>MESEQLFHRGYYRNSYNSITSASSDEELLDGAGAIMDFQTSEDDNLLDGDTAAGTHYTMTNGGSINSSTHLLDLLDEPIPGVGTYDDFHTIDWVREKCKDRERHRRINSKKKESAWEMTKSLYDAWSGWLVVTLTGLASGALAGLIDIAADWMTDLKEGICLSALWYNHEQCCWGSNETTFEERDKCPQWKTWAELIIGQAEGPGSYIMNYIMYIFWALSFAFLAVSLVKVFAPYACGSGIPEIKTILSGFIIRGYLGKWTLMIKTITLVLAVASGLSLGKEGPLVHVACCCGNIFSYLFPKYSTNEAKKREVLSAASAAGVSVAFGAPIGGVLFSLEEVSYYFPLKTLWRSFFAALVAAFVLRSINPFGNSRLVLFYVEYHTPWYLFELFPFILLGVFGGLWGAFFIRANIAWCRRRKSTKFGKYPVLEVIIVAAITAVIAFPNPYTRLNTSELIKELFTDCGPLESSSLCDYRNDMNASKIVDDIPDRPAGVGVYSAIWQLCLALIFKIIMTVFTFGIKVPSGLFIPSMAIGAIAGRIVGIAVEQLAYYHHDWFIFKEWCEVGADCITPGLYAMVGAAACLGGVTRMTVSLVVIVFELTGGLEYTVPLMAAVMTSKWVGDAFGREGIYEAHIRLNGYPFLDAKEEFTHTTLAADVMRPRRSDPPLAVLT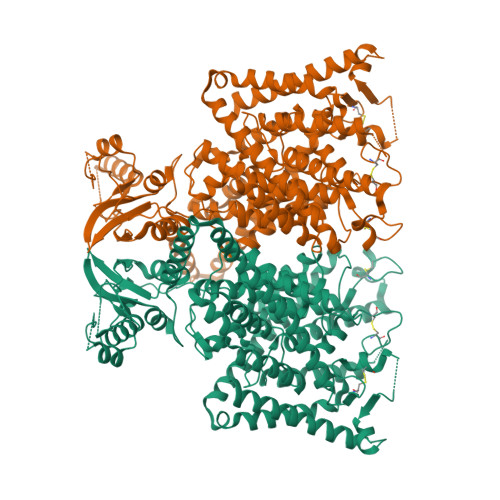QDNMTVDDIENMINETSYNGFPVIMSKESQRLVGFALRRDLTIAIESARKKQEGIVGSSRVCFAQHTPSLPAESPRPLKLRSILDMSPFTVTDHTPMEIVVDIFRKLGLRQCLVTHNGRLLGIITKKDILRHMAQTANQDPASIMFN[2x]> MRTFFVGGNWKANPKTVEEAEKLIEMLNGAKVEGNVEVVVAAPFFFLPTLQQKLRKDWKVSAENVFTKPNGAFTGEVTVPMIKSFGIEWTILGHSERRDILKEDD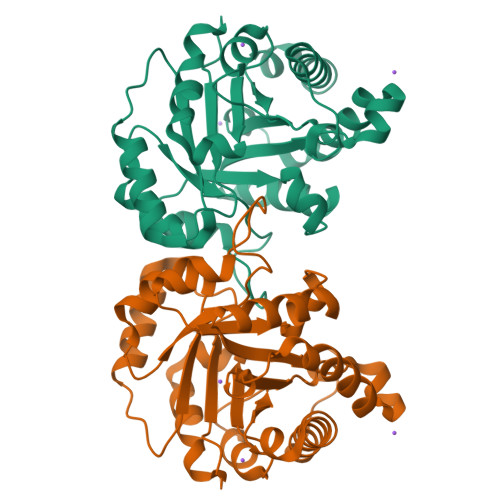EFLAAKAKFALENGMKIIYCCGEHLSEREAGKASEFVSAQIEKMIPAIPAGKWDDVVIAYEPIWAIGTGKVASTQDAQEMCKVIRDILAAKVGADIANKVRILYGGSVKPNNCNELAACPDVDGFLVGGASLEPGFINIVNSNVHSK> MGSSHHHHHHSQDPDINNKARIHWACRRGMRELDISIMPFFEHEYDSLSDDEKRIFIRLLECDDPDLFNWLMNHGKPADAELEMMVRLIQTRNRERG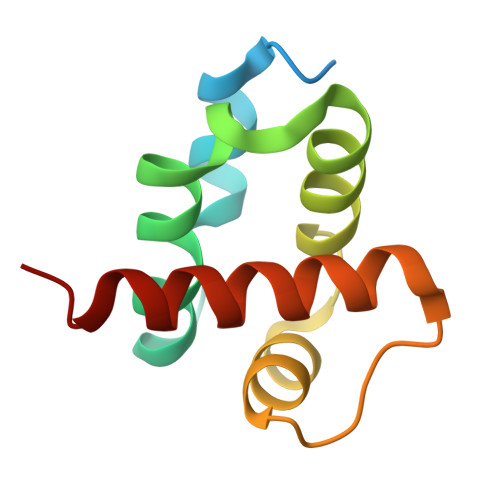PVAI>[4x]MAAINTKVKKAVIPVAGLGTRMLPATKAIPKEMLPLVDKPLIQYVVNECIAAGITEIVLVTHSSKNSIENHFDTSFELEAMLEKRVKRQLLDEVQSICPPHVTIMQVRQGLAKGLGHAVLCAHPVVGDEPVAVILPDVILDEYESDLSQDNLAEMIRRFDETGHSQIMVE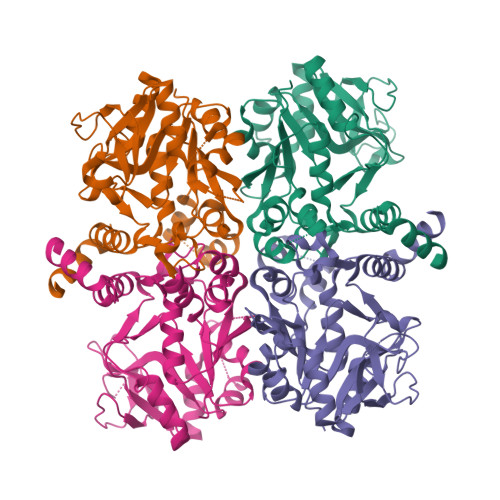PVADVTAYGVVDCKGVELAPGESVPMVGVVEKPKADVAPSNLAIVGRYVLSADIWPLLAKTPPGAGDEIQLTDAIDMLIEKETVEAYHMKGKSHDCGNKLGYMQAFVEYGIRHNTLGTEFKAWLEEEMGIKK>[2x]MNIHEWQSKQLIQKYGGRAQSGEVAFSPERSRDIAKKLWNQFPGCKFVVKAQVLAGGRGKGH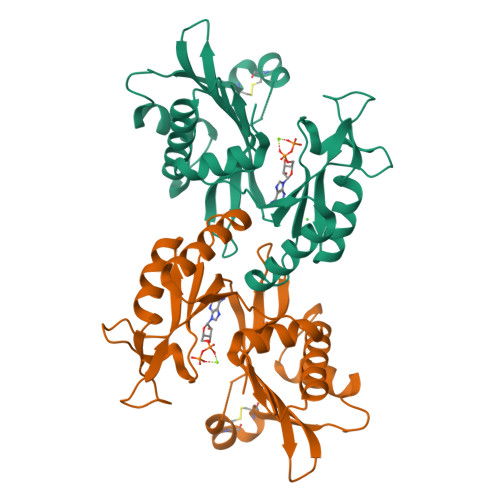WEHGMQGGVKLAKTPEEVYEIANEMIGHKLITKQTGAKGINCNKVMVCGAVDILKEFYLSILLDRAMGCPVIIATSQGGMGIEEVAQKCPECLFKVPISVKNGPTNEQLVKLAKDLGLEGDLVQDCVDNVKALYQVFDKCDSTMVEINPLGVIETPTDEKVICCLDAKIAFDKDAAFGLEHHHHHHHH> MSLRRGIYHIENAGVPSAIDLKDGSSSDGTPIVGWQFTPDTINWHQLWLAEPIPNVADTFTLCNLFSGTYMDLYNGSSEAGTAVNGWQGTAFTTNPHQLWTIKKSSDGTSYKIQNYGSKTFVDLVNGDSSDGAKIAGWTGTWDEGNPHQKWYFNRMSVSSAEAQAAIARNPHIHGTYRGYILDGEYLVLPNATFT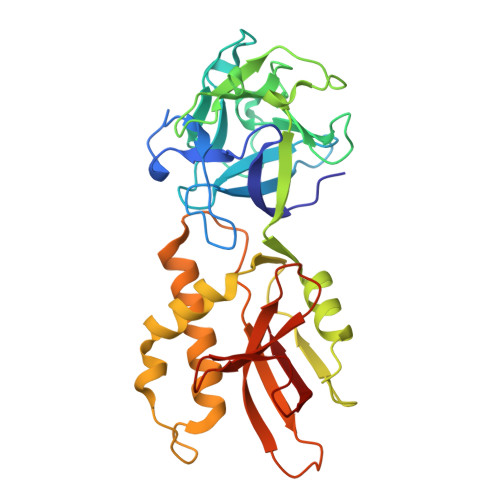QIWKDSGLPGSKWREQIYDADDFAIAMKAAVGKWGADSWKANGFAIFCGVMLGVNKAGDAAHAYNFTLTKDHADIVFFEPQNGGYLNDIGYDSYMAFY>[2x]TKPLDGINVLDFTHVQAGPACTQMMGFLGANVIKIERRGSGDMTRGWLQDKPNVDSLYFTMFNCNKRSIELDMKTPEGKELLEQMIKKADVMVENFGPGALDRMGFTWEYIQELNPRVILASVKGYAEGHANEHLKVYENVAQCSGGAAATTGFWDGPPTVSGAALGSSNSGMHLMIGILAALEIRH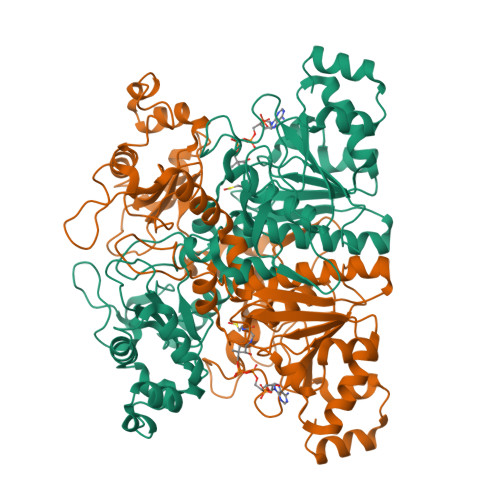KTGRGQKVAVAMQDAVLNLVRIKLRDQQRLERTGILAEYPQAQPNFAFDRDGNPLSFDNITSVPRGGNAGGGGQPGWMLKCKGWETDADSYVYFTIAANMWPQICDMIDKPEWKDDPAYNTFEGRVDKLMDIFSFIETKFADKDKFEVTEWAAQYGIPCGPVMSMKELAHDPSLQKVGTVVEVVDEIRGNHLTVGAPFKFSGFQPEITRAPLLGEHTDEVLKELGLDDAKIKELHAKQVV3-[1-[(3-methoxyphenyl)methyl]indol-6-yl]-1~{H}-pyrazol-5-amine | C19 H18 N4 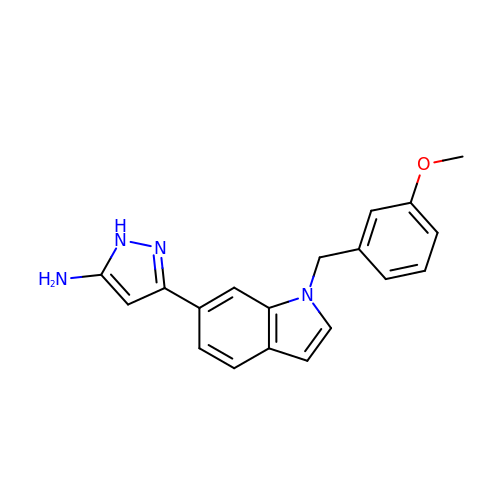O | HOUGYQANDNDSLX-UHFFFAOYSA-N>[8x]MSAAEGAVVFSEEKEALVLKSWAIMKKDSANLGLRFFLKIFEIAPSARQMFPFLRDSDVPLETNPKLKTHAVSVFVMTCEAAAQLRKAGKITVRETTLKRLGGTHLKYGVADGHFEVTR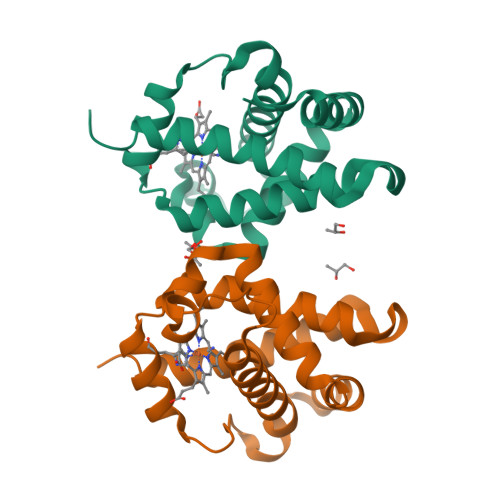FALLETIKEALPADMWGPEMRNAWGEAYDQLVAAIKQEMKPAE> KQTA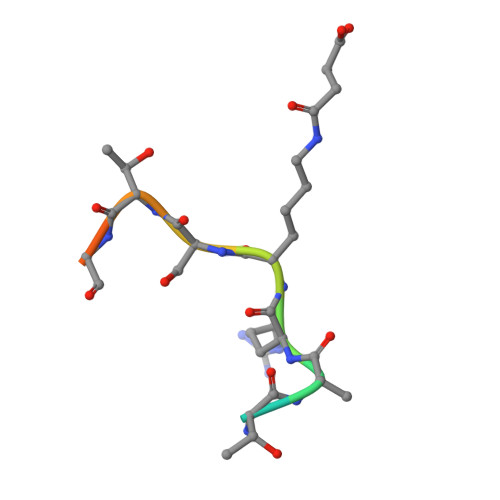RXSTGGKA> GPRSQKQLELKVSELVQFLLIKDQKKIPIKRADILKHVIGDYKDIFPDLFKRAAERLQYVFGYKLVELEPKSNTYILINTLEPVEEDAEMRGDQGTPTTGLLMIVLGLIFMKGNTLKETEAWDFLRRLGVYPTKKHLIFGDPKKLITEDFVRQRYLEYRRIPHTDPVDYEFQWGPRTNLELSKMKVLKFVA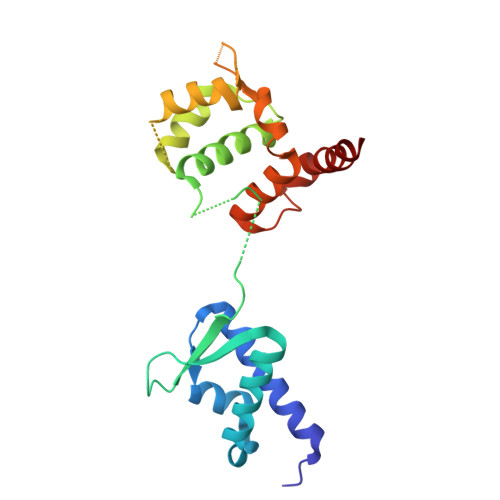KVHNQDPKDWPAQYCEALADEENRAR> AESTLGAAAAQSGRYFGTAIASGKLGDSAYTTIASREFNMVTAENEMKIDATEPQRGQFNFSAGDRVYNWAVQNGKQVRGHTLAWHSAQPGWMQSLSGSTLRQAMIDHINGVMGHYKGKIAQWDVVNEAFSDDGSGGRRDSNLQRTGNDWIEVAFRTARAADPAAKLCYNDYNIENWTWAKTQGVYNMVRDFKQRGVPIDCVGFQSHFNSGSPYNSNFRTTLQNFAALGVDVAITELDIQGASSSTYAAVTNDCLAVSRCLGITVWGVRDTDSWASGDTPLLF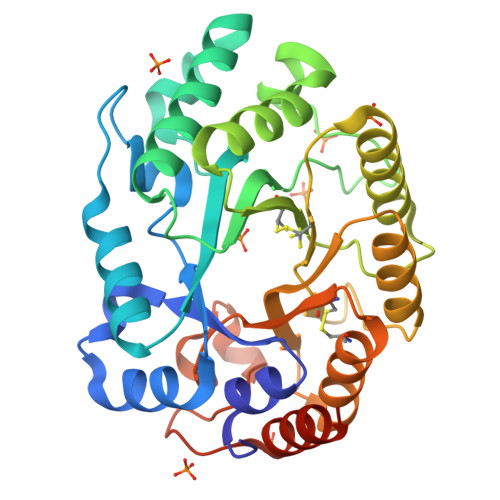NGDGSKKAAYTAVLNALNGGGSRSHHHHHH>[2x]PTYPKYL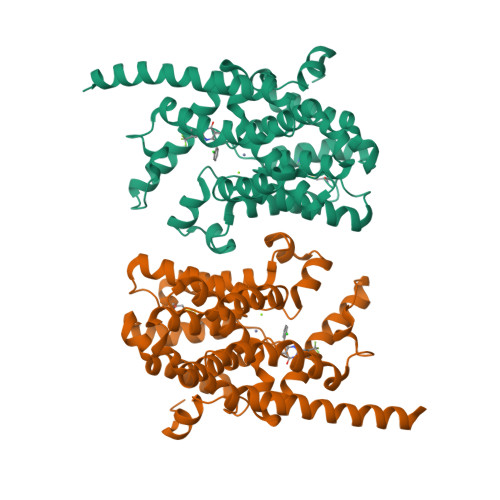LSPETIEALRKPTFDVWLWEPNEMLSCLEHMYHDLGLVRDFSINPVTLRRWLFCVHDNYRNNPFHNFRHCFCVAQMMYSMVWLCSLQEKFSQTDILILMTAAICHDLDHPGYNNTYQINARTELAVRYNDISPLENHHCAVAFQILAEPECNIFSNIPPDGFKQIRQGMITLILATDMARHAEIMDSFKEKMENFDYSNEEHMTLLKMILIKCCDISNEVRPMEVAEPWVDCLLEEYFMQSDREKSEGLPVAPFMDRDKVTKATAQIGFIKFVLIPMFETVTKLFPMVEEIMLQPLWESRDRYEELKRIDDAMKELQKK N-[(3M)-3-(6-methoxypyridin-3-yl)benzene-1-sulfonyl]-L-cysteinamide | C15 H17 N3 O4 S2 | 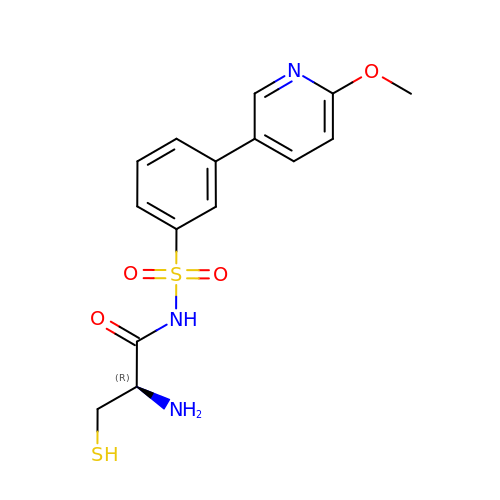LQDUHWTWGXAMOC-ZDUSSCGKSA-N>AERTMFYGKGDVYVFRTYANPLKGLKQIPESNFTEKHNTIFGMNAKVALKGEQLLTSFTEGDNSLVVATDSMKNFIQRHAASYEGATLEGFLQYVCEAFLAKYSHLDAVRLEAKEYAFDDIQVGTDKGVVTSDLVFRKSRNEYVTATVEVARTASGTEVVEQASGIADIQLIKVSGSSFYGYIIDEYTTLAEATDRPLYIFLNIGWAYENQDDAKGDNPANYVAAEQ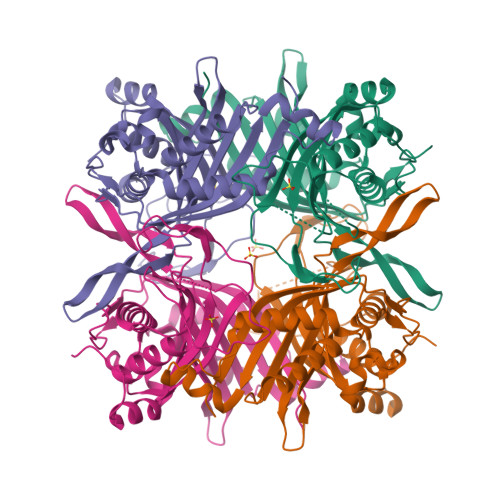VRDIAASVFHTLDNKSIQHLIYHIGLTILDRFPQLTEVNFGTNNRTWDTVVEGTDGFKGAVFTEPRPPFGFQGFSVHQEDLAREKASANSEYVALKLAAALKHHHHHH[4x]> GSHMAIDTYEFASDAERERFRNLTQELRCPKC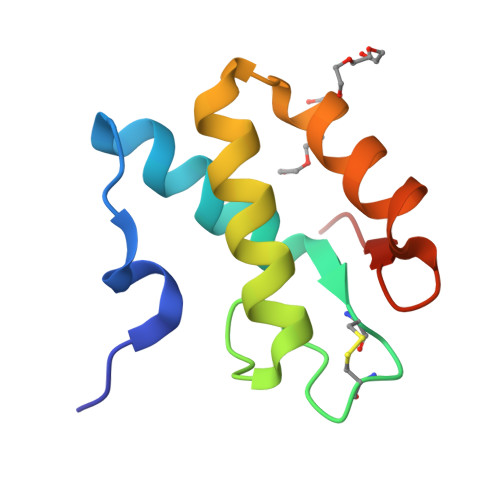QNQDIADSNAPIAADLRKQIYGQLQQGKSDGEIVDYMVARYGDFVRYKPPVN2-[(1S)-1-({6-amino-5-[(1H-pyrazol-4-yl)ethynyl]pyrimidin-4-yl}amino)ethyl]-5-chloro-3-phenylquinazolin-4(3H)-one 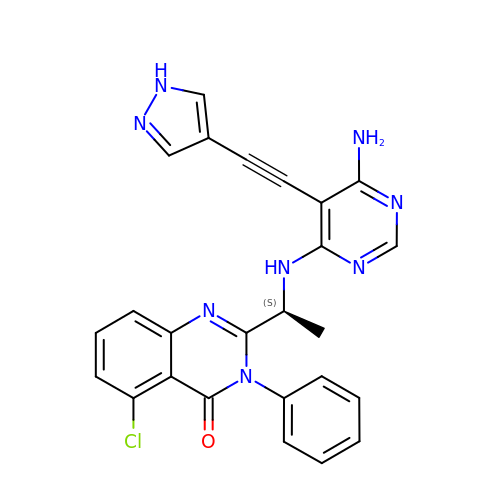| C25 H19 Cl N8 O | QSVWZWFVMMFIJE-HNNXBMFYSA-N> IVGGTSASAGDFPFIVSISRNGGPWCGGSLLNANTVLTAAHCVSGYAQSGFQIRAG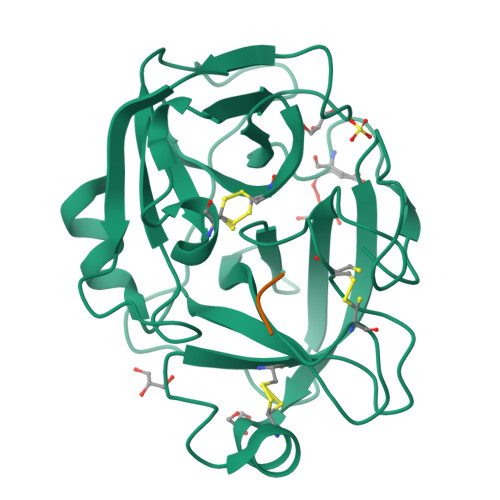SLSRTSGGITSSLSSVRVHPSYSGNNNDLAILKLSTSIPSGGNIGYARLAASGSDPVAGSSATVAGWGATSEGGSSTPVNLLKVTVPIVSRATCRAQYGTSAITNQMFCAGVSSGGKDSCQGDSGGPIVDSSNTLIGAVSWGNGCARPNYSGVYASVGALRSFIDTYA;> GAK The enzyme inorganic pyrophosphatase (PPase) catalyzes the hydrolysis of pyrophosphate (PPi) to inorganic phosphate (Pi). This is an exergonic reaction and can be coupled to several unfavorable and energy demanding biochemical transformations such as DNA replication, protein synthesis and lipid metabolism. Family I PPases are Mg2+ dependent enzymes known to exist as homo-hexamers in prokaryotes and dimers in eukaryotes. We report structural and biochemical characterization of these two apicomplexan PPases.

The TgPPase crystal structure was refined to 2.35 Å and showed the same structural overall fold as PfPPase. However, TgPPase lacked both N- and C-terminal regions and the structure contains residues 74–308, most likely due to proteolysis of N-terminal region during crystallization. In contrast to PfPPase, the active site of TgPPase contained two bound Mg2+ ions. One Mg2+ was bound at M1 site coordinated by Asp190, Asp195 and Asp227. The Mg2+ was bound to protein in M2 site predominantly through water molecules and Asp195. However, no electron density for either Pi or PPi was observed in the TgPPase active site despite addition of PPi during crystallization. Therefore, it is feasible that the observed conformation in the active site represents a state where both Pis have already dissociated. Like PfPPase, TgPPase also formed dimers in solution and in the crystal. Two TgPPase subunits buried 1780 Å2 (50%) of total ASA and are held together mainly by a network hydrogen bonds and Van der Waal forces. On the other hand, TgPPase monomers are joined by α3 only.

>[2x]VYRRLVSGTEGEKDFRVLLSKKSGERLSPWHDIPLFPNGRDARPLLFNMVVEIPKNTRRKMEMQLRLPFTPIMQDLKKDGSLREYASTLYWNYGAFPQTWEDPREPGGREVFHARGDGDPLDVVEIGSEVLPVGGVVPVKVLGALAMIDGGELDWKVLAIREGDPLFSQLNSVADVERLCRGVVPGIREWFRWYKLPTDNVVNQFGHDEAALPAADAERVVYRAHEHYLRLLSEE~{N}-(5-chloranylpyridin-2-yl)-4-pyridin-2-yl-1,3-thiazol-2-amine 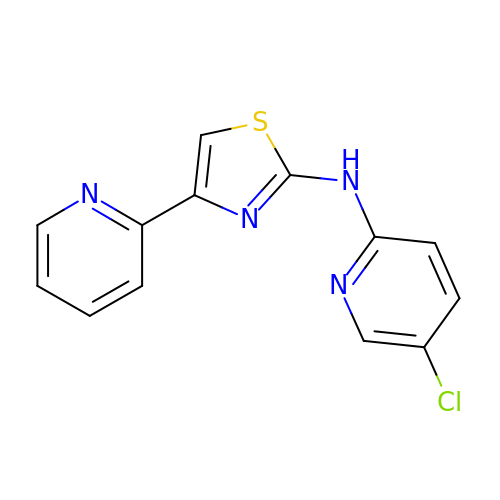| C13 H9 Cl N4 S | XIMLXPRKZACEAD-UHFFFAOYSA-N2-hydroxyethyl 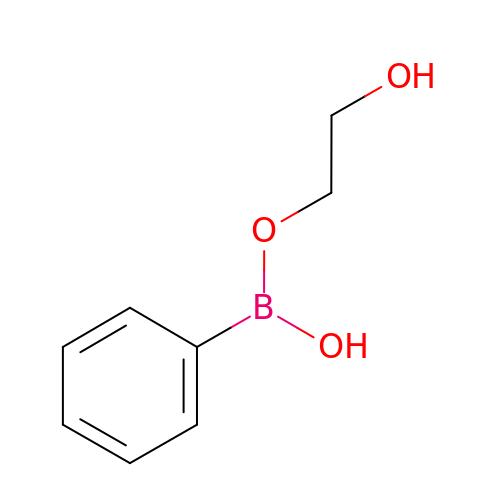hydrogen phenylboronate | C8 H11 B O3 | MCBDCMMJWCRCFZ-UHFFFAOYSA-N> MSDTNYAVIYDLHSHTTASDGCLTPEALVHRAVEMRVGTLAITDHDTTAAIAPAREEISRSGLALNLIPGVEISTVWENHEIHIVGLNIDITHPLMCEFLAQQTERRNQRAQLIAERLEKAQIPGALEGAQRLAQGGAVTRGHFARFLVECGKASSMADVFKKYLARGKTGYVPPQWCTIEQAIDVIHHSGGKAVLAHPGRYNLSAKWLKRLVAHFAEHHGDAMEVAQCQQSPNERTQ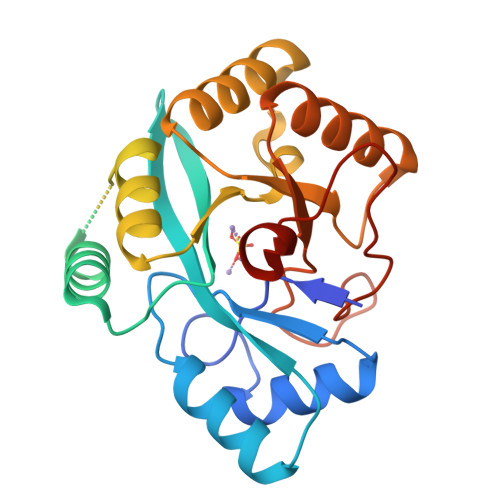LAALARQHHLWASQGSDFHQPCPWIELGRKLWLPAGVEGVWQLWEQPQNTTEREL>SWQTYVDTNLVGTGAVTQAAIIGHDGNTWATSAGFAVSPANGAALANAFKDATA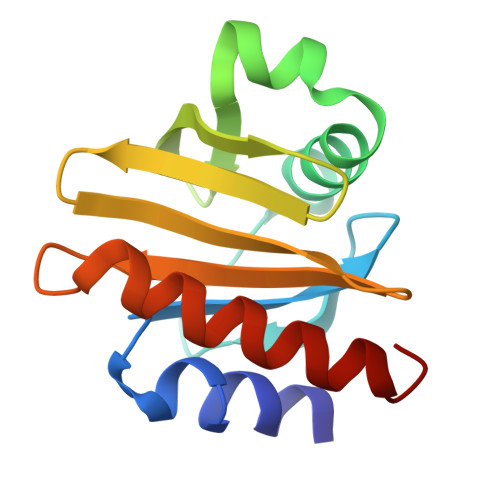IRSNGFELAGTRYVTIRADDRSVYGKKGSAGVITVKTSKAILIGVYNEKIQPGTAANVVEKLADYLIGQGF[2x]> GSHMRKIQRYVRKDG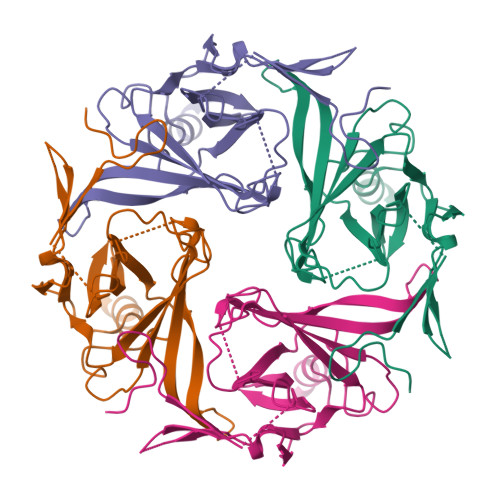KCNVHHGNVREKRAETLVFSTHAVISMRDGKLCLMFRVGDLRNSHIVEASIRAKLIKSKQTSEGEFIPLNQTDINVGYYTGDDRLFLVSPLIISHEINQQSPFWEISKAQLPKEELEIVVILEGMVEATGMTCQARSSYITSEILWGYRFTPVLTLEDGFYEVDYNSFHETYETSTPSLSAKELAELANRAEV> GSDEKRLHFGNGHLKLPGLRTFVDPHTYEDPTQTVHEFAKELDATNISIDKVVGAGEFGEVCSGRLKLPSKKEISVAIKTLKVGYTEKQRRDFLGEASIMGQFDHPNIIRLEGVVTKSKPVMIVTEYMENGSLDS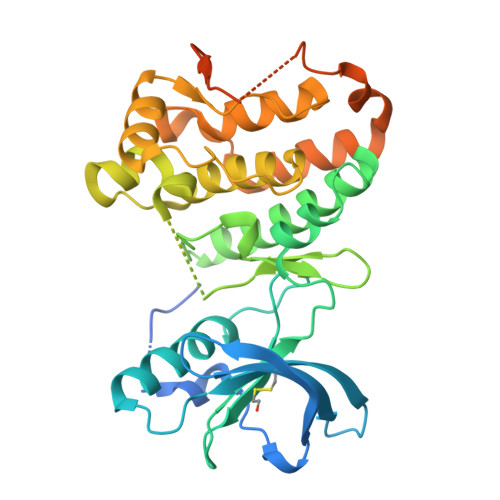FLRKHDAQFTVIQLVGMLRGIASGMKYLSDMGYVHRDLAARNILINSNLVCKVSDFGLSRVLEDDPEAAYTTRGGKIPIRWTSPEAIAYRKFTSASDVWSYGIVLWEVMSYGERPYWEMSNQDVIKAVDEGYRLPPPMDCPAALYQLMLDCWQKDRNNRPKFEQIVSILDKLIRNPGSLKIITSAAARPSNLLLDQSNVDITTFRTTGDWLNGVWTAHCKEIFTGVEYSSCDTIAKIS> QECTKFKVSSCRECIESGPGCTWCQKLNFTGPGDPDSIRCDTRPQLLMRGCAADDIMDPTSLAETQEDHNGGQKQLSPQKVTLYLRPGQAAAFNVTFRRAKGY;> SRVFLDHNALPDTLKVTYDSFCSNGVTHRNQPRGDCDGVQINVPITFQVKVTATECIQEQSFVIRALGFTDIVTVQVLPQCECRCRDQSRDRSLCHGKGFLECGICRC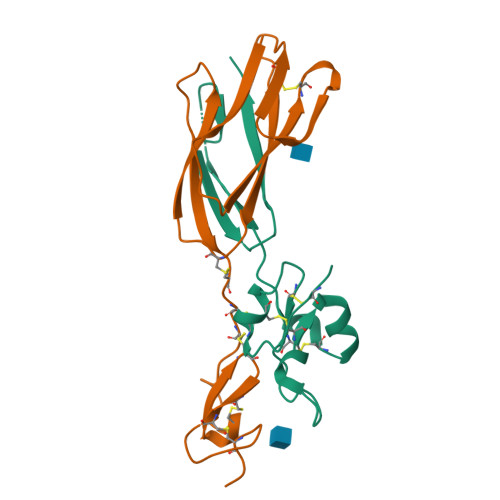DTGYIGKNCEHH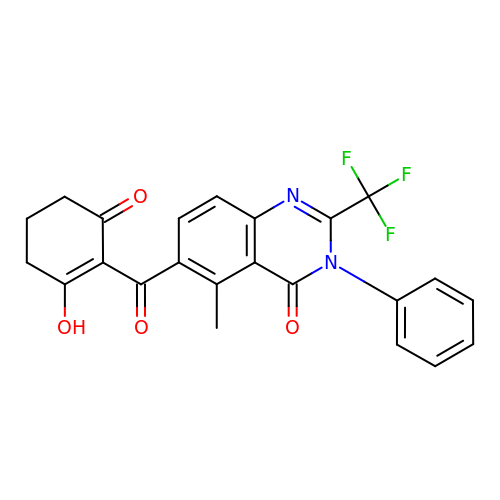5-methyl-6-(2-oxidanyl-6-oxidanylidene-cyclohexen-1-yl)carbonyl-3-phenyl-2-(trifluoromethyl)quinazolin-4-one | C23 H17 F3 N2 O4 | GGGBHWJELOCVAB-UHFFFAOYSA-N> QFWDLNAKLVDIPTKMRVERWAFNFSELIRDPKGRQSFQHFLRKEFSGENLGFWEACEDLKYGDQSKVKEKAEEIYKLFLAPGARRWIN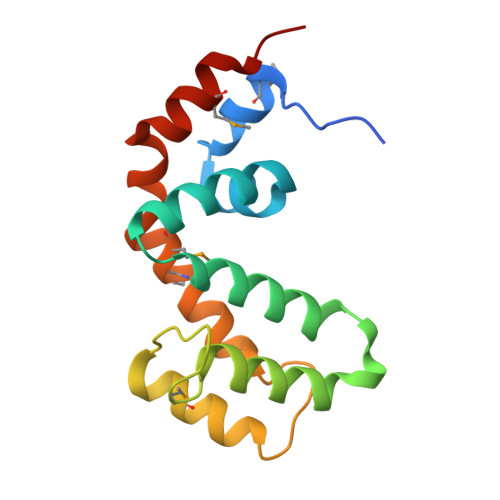IDGKTMDITVKGLKHPHRYVLDAAQTHIYMLMKKDSYARYLKSPIYKEMLAKAIEPQG>[2x]MNGSIQGKPLLGKGMSES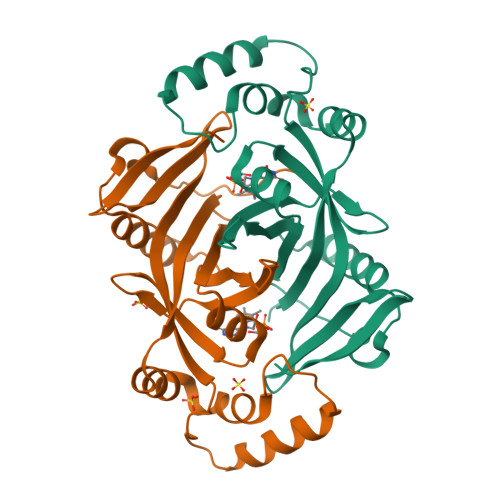LTGTLDAPFPEYQTLPADPMSVLHNWLERARRVGIREPRALALATADSQGRPSTRIVVISEISDAGVVFSTHAGSQKGRELLHNPWASGVLYWRETSQQIILNGQAVRLPNAKADDAWLKRPYATHPMSSVSRQSEELQDVQAMRNAARQLAELQGPLPRPEGYCVFELRLESLEFWGNGQERLHERLRYDRSDTGWNVRRLQP> 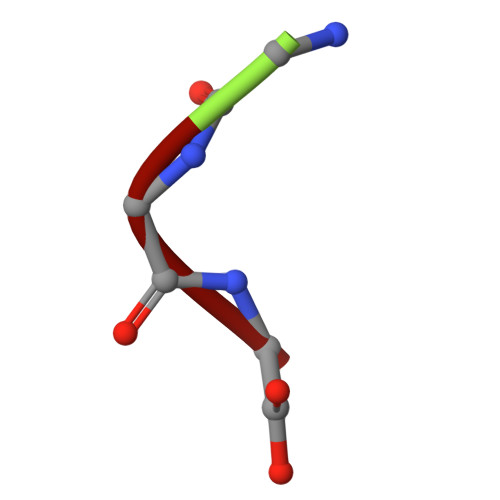GGG> ETGCNKALCASDVSKCLIQELCQCRPGEGNCSCCKECMLCLGALWDECCDCVGMCNPRNYSDTPPTSKSTVEELHEPIPSLFRALTEGDTQLNWNIVSFPVAEELSHHENLVSFLETVNQPHHQNVSVPSNNVHAPYSSDKEHMCTVVYFDDCMSIHQCKISCESMGASKYRWFHNACCECIGPECIDYGSKTVKCMNCMFGTKHHHHHH

Twisted gastrulation (TWSG1) is an evolutionarily conserved secreted glycoprotein which controls signaling by Bone Morphogenetic Proteins (BMPs). TWSG1 binds BMPs and their antagonist Chordin to control BMP signaling during embryonic development, kidney regeneration and cancer. TWSG1 is composed of two distinct, disulfide-rich domains. The TWSG1 N-terminal domain occupies the BMP type 1 receptor binding site on BMPs, whereas the C-terminal domain binds to a Chordin family member.

TWSG1 crystallized as a dimer in the asymmetric unit, an arrangement that we observed in two crystal forms. The structure of TWSG1 reveals a modular architecture, comprising an α-helical N-terminal domain (NTD, Cys26–Arg80) connected by an extended 18 Å-long linker to a mixed-α/β C-terminal domain (CTD, Pro87–Phe223). The NTD of TWSG1 folds into a compact bundle of three α-helices locked by 7 disulfides. The CTD of TWSG1 is stabilized by 5 disulfide bonds (VIII–XII) and contains a sheet comprised of 5 antiparallel β-strands which constitute its core. Search of structural homologs among all previously determined structures in the Protein Data Bank (PDB) did not yield any hits highlighting TWSG1’s unique structural folds and their arrangement. Remarkably, a relatively small NTD of ~50 amino acid residues contains 7 disulfide bonds and thus serves as a stable, rigid scaffold suitable to mediate TWSG1 interactions with its binding partners.(2E)-3-{7-[(1S)-1-(2,6-dichloro-3-fluorophenyl)ethoxy]-1-methylnaphthalen-2-yl}prop-2-enoic acid | C22 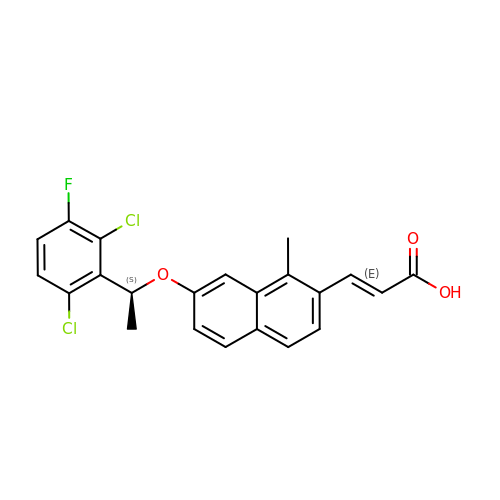H17 Cl2 F O3 | RHZRLFIWQWRTKH-PPOCWRSBSA-N>[2x]GAEIPKEMLRAQTNXILRNVLKQGDNYVYGIIKQVKEASNGEMELNEATLYTIFKRLEKDGIISSYWGDESQGGRRKYYRLTEIGHENNRLAFEGWSRVDKIIENLEANKKSEAIKSRWSHPQFEK

Our group previously produced a promiscuous designer enzyme by incorporating the noncanonical amino acid para-aminophenylalanine at position valine-15 of the Lactococcal multidrug resistance regulatory (LmrR) protein scaffold. In doing so, we enabled the formation of iminium ion intermediates formed by the condensation of aldehydes with the amino moiety of the pAF catalytic residue, thus mimicking known reactivities of small molecule organocatalysts in a protein scaffold. Assessment of the Michaelis–Menten kinetic parameters of these evolved mutants revealed that the mutations that improved one catalytic activity caused a concomitant decrease in the other, i.e., directed evolution produced catalytic specialization. We successfully obtained crystals for both the RGN and RMH mutants, with one crystal diffracting to a maximum resolution of 2.45 Å for the former mutant and two crystals diffracting at 2.55 and 2.24 Å for the latter.

Comparing the structure of LmrR_pAF16 with the RGN mutant reveals an unexpected change in the quaternary structure. With only three mutations, the assembly of the monomers to form the homodimeric structure is markedly different, as seen in 3D-structural alignments. This is also reflected in a closing of the hydrophobic pocket formed at the dimer interface, where the distance between the two closest atoms of the W96/W96′ side chains decreases from 6.3 Å in LmrR_pAF to 4.0 Å in the RGN mutant. Accordingly, the pocket volume of the RGN mutant (∼800 Å3), as estimated using PyVOL,21 is around half that of LmrR_pAF (∼1600 Å3). The newly installed R18 side chain forms hydrogen bonds with carbonyl moieties in the N88 and N89 side chains (the latter was also introduced in directed evolution). In one monomer, the H-bonding partner of R18 is E7′ rather than N88/N89; this interaction also likely affects the dimer assembly and hence the pocket volume. These new interactions may “pin” together the α1 and α4 helices and thus provide the large increase in angle, from 51.5° and 52.7° for each monomer LmrR_pAF to 54.5° and 60.1° for each monomer in the RGN mutant, which in turn allows tighter packing of the two monomers to form the homodimer affording the resulting smaller pocket volume. We also observed an increase in proximity between α1 and α4′ helices (i.e., between two monomers forming the homodimer), which may be caused by increased space afforded for the Q12 side chain by the S95G mutant in RGN, allowing for closer packing of these helixes and gives a decreased distance between the α-carbons of these residues by almost 1 Å compared to LmrR_pAF. Strikingly, in the RGN variant the 2-methyl-indole substrate remained in the pocket for five of the six replicates, with a clear bias toward dihedral angles indicative of the formation of the experimentally verified (S)-enantiomer upon close approaches.> MRVLLIHADYFEYEVKDKALKNPEPISEDMKRGRMEEVLVAFISVEKVDEKNPEEVSLKAIEEISKVAEQVKAENVFVIPWAHLSSELAKPSVAMDILNRVYQGLKERGFNVGKAPFGYYIAAKISCK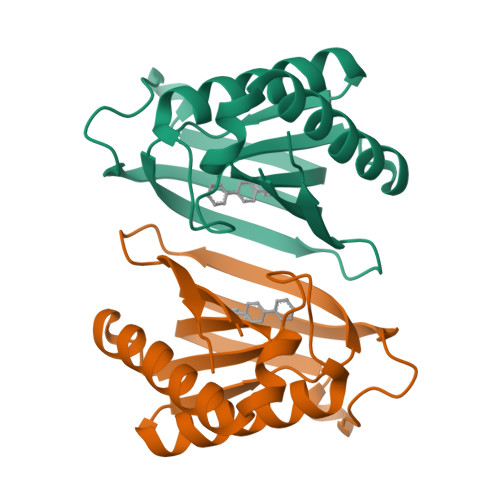GHPLAELSRTIVPEELEHHHHHH>[4x]MHHHHHHEPLILTAAITGAETTRADQPNLPITPEEQAKEAKACFEAGARVIHLHIREDDGRPSQRLDRFQEAISAIREVVPEIIIQISTGGAVGESFDKRLAPLALKPEMATLNAGTLNFGDDIFINHPADIIRLAEAFKQYNVVPEVEVYESGMVDAVARLIKKGIITQNPLHIQFVLGVPGGMSGKPKNLMYMMEHLKEEIPTATWAVAGIGRWHIPTSLIAMVTGGHIRCGFEDN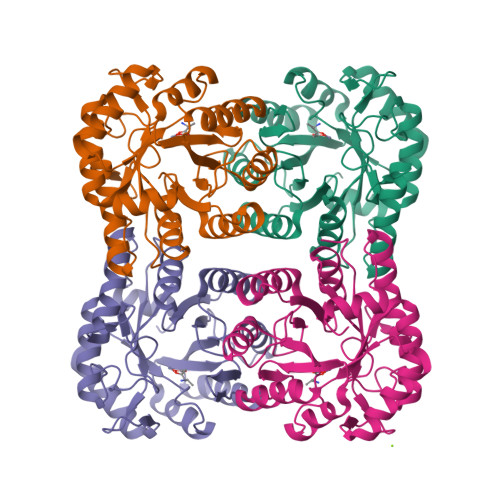IFYHKGVIAESNAQLVARLARIAKEIGRPLATPEQAREILALNK> MKTAALFVSKEFEEEAIALVEGANYKVTSIYKLPKSPNVKFYIQYDKLQQIKNDEEISTLIIFEQLKPRHFINIRRELKGKEVLDKILLLLEIFALHAGSKEAKMQIELARLKYELPIIKETYTKSKIGEQQGPLGAGTYGVESTIKFYKRRINKLMKELESIKIFKEKSIESNKRNNIPSIGIVGYTNSGKTSLFNSLTGLTQKVDTKLFTTMSPKRYAIPINNRKIMLVDTVGFIRGIPPQIVDAFFVTLSEAKYSDALILVIDSTFSENLLIETLQSSFEILREIGVSGKPILVTLNKIDKINGDLYKKLDLVEKLSKELYSPIFDVIPISALKRTNLELLRDKIYQLATQLSLEHHHH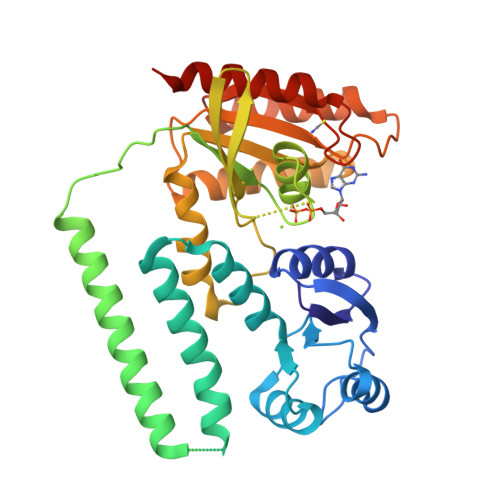HH>[2x]MSETPLLDELEKGPWPSFVKEIKKTAELMEKAAAEGKDVKMPKGARGLLKQLEISYKDKKTHWKHGGIVSVVGYGGGVIGRYSDLGEQIPEVEHFHTMRINQPSGWFYSTKALRGLCDVWEKWGSGLTNFHGSTGDIIF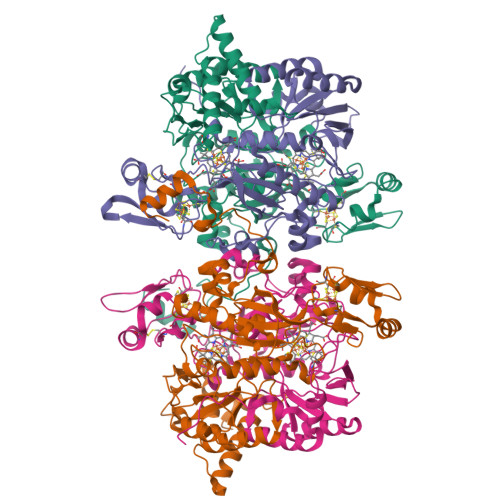LGTRSEYLQPCFEDLGNLEIPFDIGGSGSDLRTPSACMGPALCEFACYDTLELCYDLTMTYQDELHRPMWPYKFKIKCAGCPNDCVASKARSDFAIIGTWKDDIKVDQEAVKEYASWMDIENEVVKLCPTGAIKWDGKELTIDNRECVRCMHCINKMPKALKPGDERGATILIGGKAPFVEGAVIGWVAVPFVEVEKPYDEIKEILEAIWDWWDEEGKFRERIGELIWRKGMREFLKVIGREADVRMVKAPRNNPFMFFEKDELKPSAYTEELKKRGMW;>[2x]MVVEGVKTDFGPPYFRDLLHPVIAKNYGKWKYHEVVKPGVIKRVAESGDVIYVVRFGTPRLLSIYTVRELCDIADKYSDGYLRWTSRNNVEFFVTDESKIDDLINEVQERVGFPCGGTWDAVKGEYGLSNIVHTQGWIHCHTPAIDASGIVKAVMDELYEYFTDHKLPAMCRISLACCANMCGAVHASDIAIVGIHRTPPIPNDEAIRKTCEIPSTVAACPTGALKPDMKNKTIKVDVEKCMYCGNCYTMCPGMPLFDPENDGAAIMVGGKLSEARRMPELSKVVVPWVPNEPPRWPTLVKYVKQILEAWAANANKHERLIEWVDRIGWERFFELTGLEFTQHLIDDYRITPYFYSEFRASTQFKW> MALVPVGMAPRQMRVNRCIFASIVSFDACITYKSPCSPDAYHDDGWFICNNHLIKRFKMSKMVLPIFDEDDNQFKMTIARHLVGNKERGIKRILIPSATNYQDVFNLNSMMQAEQLIFHLIYNNENAVNTICDNLKYTEGFTSNTQRVIHSVYATTKSILDTTNPNTFCSRVSRDELRFFDVTNARALRGGAGDQLFNNYSG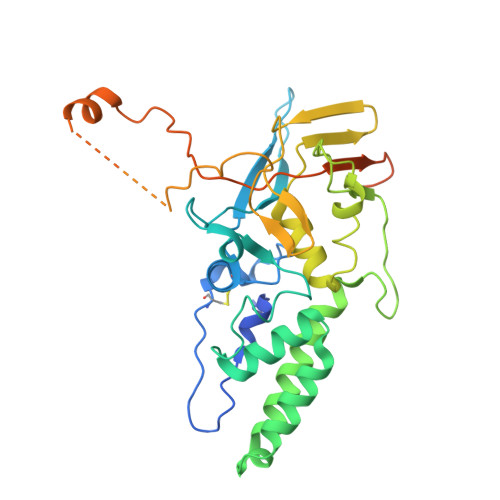FLQNLIRRAVAPEYLQIDTEELRFRNCATCIIDETGLVASVPDGPELYNPIRSSDIMRSQPNRLQIRNVLKFEGDTRELDRTLSGYEEYPTYVPLFLGYQIINSENNFLRNDFIPRANPNATLGGGAVAGPAPGVAGEAGGGIAV>[8x]MVMQLKSRVFIVTGASSGLGAAVTRMLAQEGATVLGLDLKPPAGEEPAAELGAAVRFRNADVTNEADATAALAFAKQEFGHVHGLVNCAGTAPGEKILGRSGPHALDSFARTVAVNLIGTFNMIRLAAEVMSQGEPDADGERGVIVNTASIAAFDGQIGQAAYAASKGGVAALTLPAARELARFGIRVVTIAPGIFDTPMMAGMPQDVQDALAASVPFPPRLGRAEEYAAL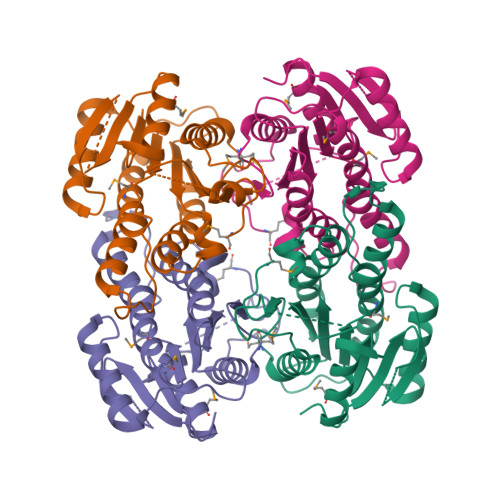VKHICENTMLNGEVIRLDGALRMAPR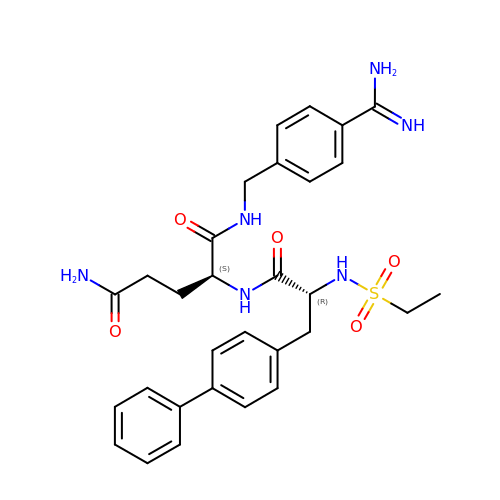2-(3-BIPHENYL-4-YL-2-ETHANESULFONYLAMINO-PROPIONYLAMINO)-PENTANEDIOIC ACID 5-AMIDE 1-(4-CARBAMIMIDOYL-BENZYLAMIDE) | C30 H36 N6 O5 S | DSXLGZNVVMZNSK-IZZNHLLZSA-N> GEGK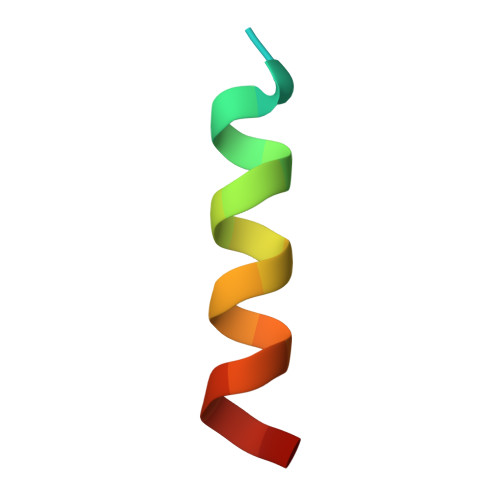EDAFSKLKEKFMNELHK>[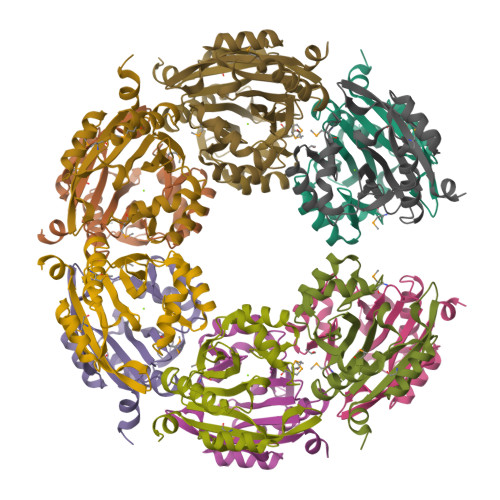6x]SNAMNSQLTLRALERGDLRFIHNLNNNRNIMSYWFEEPYESFDELEELYNKHIHDNAERRFVVEDAQKNLIGLVELIEINYIHRSAEFQIIIAPEHQGKGFARTLINRALDYSFTILNLHKIYLHVAVENPKAVHLYEECGFVEEGHLVEEFFINGRYQDVKRMYILQSKYLNRSE>MSINQLTLAVASDQEISAHGYPTMSDAVEHFSSSASHGFKDCRFVAFGLQDIVIGVEPSDFVVAL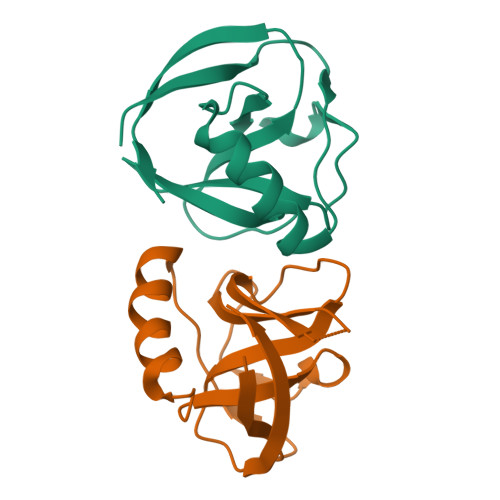EGDEILTAYIATFGARPRCLRGWLIPSNSNYVLEEFQVIFGKRGGLEHHHHHHHH[2x]>ENYGIEWHSVRDSEGQKLLIGVGPEGISICKDDFSPINRIAYPVVQMATQSGKNVYLTVTKESGNSIVLLFKMIS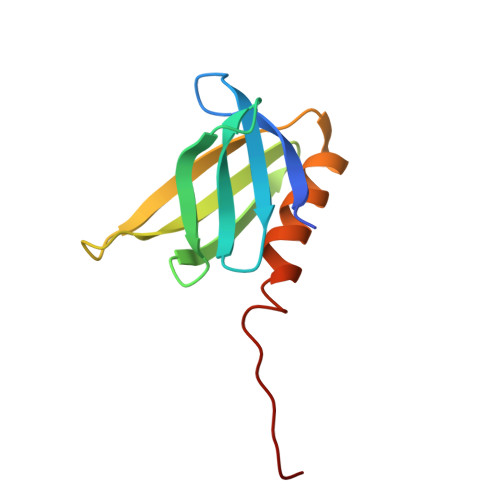TRAASGLYRAITETHAFYRCDTVTSA[3x]> XPQQ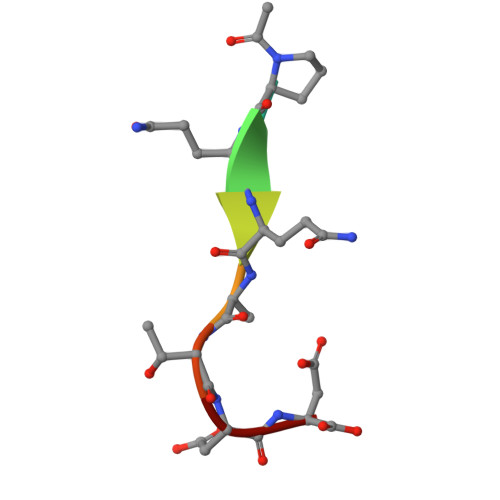ATDD>MGQIIEEKISGTKDTVDFVRNKDISGITSIKLPTVKVSES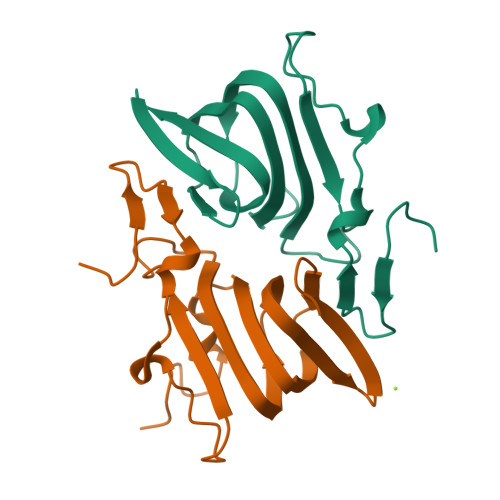DRLDTGNPSDVVYTKDLFTLEESPRLGCGMMEMKETTFDWTLNYDEIDYVIDGTLDIIIDGRKVSASSGELIFIPKGSKIQFSVPDYARFIYVTYPADWASQNLEHHHHHH[2x]(2R)-2-{[6-(4-aminopiperidin-1-yl)-3,5-dicyano-4-ethylpyridin-2-yl]sulfanyl}-2-[4-(trifluoromethyl)phenyl]acetamide | C23 H23 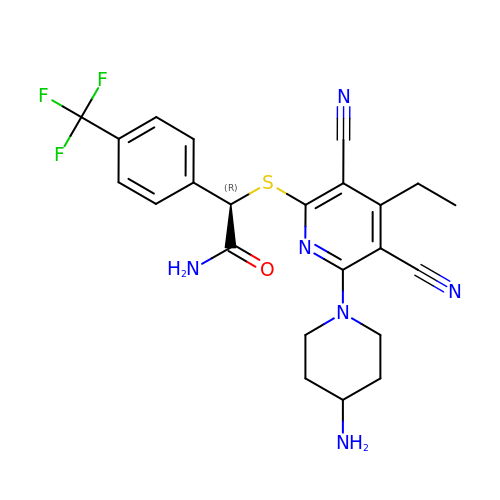F3 N6 O S | HCPBFQRBYJPHKZ-LJQANCHMSA-N> WSATNEEDDLSVEAEIAHQIAESFSKKYKFPSRSSGIFLYNFEQLKMNLDDIVKEAKNV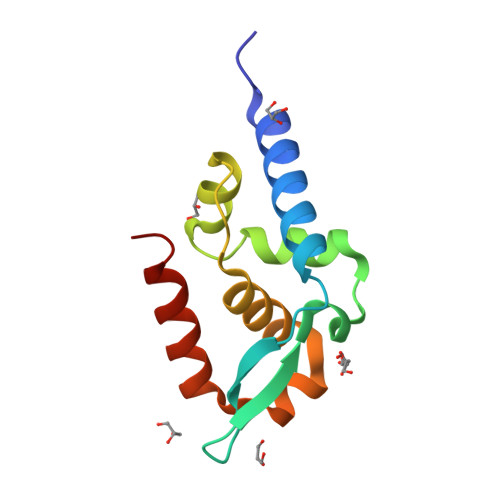PGVTRLAHDGSKIPLRCVLGWVALANSKKFQLLVEADKLSKIMQDDLNRYTSC>MDKNLHQPLGGNEMPRFGGIATMMRLPHVQSPAELDALDAAFVGVPLDIGTSLRSGTRFGPREIRAESVMIRPYNMATGAAPFDSLNVADIGDVAINTFNLLEAVRIIEQEYDRILGHGILPLTLGGDHTITLPILRAIKKKHGKVGLVHVDAHADVNDHMF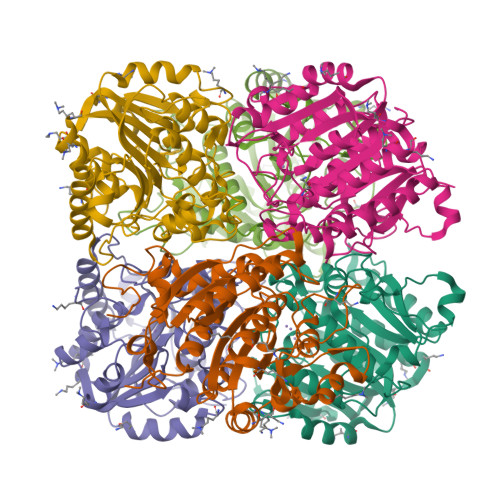GEKIAHGTTFRRAVEEDLLDCDRVVQIGLRAQGYTAEDFNWSRKQGFRVVQAEECWHKSLEPLMAEVREKVGGGPVYLSFDIDGIDPAWAPGTGTPEIGGLTTIQAMEIIRGCQGLDLIGCDLVEVSPPYDTTGNTSLLGANLLYEMLCVLPGVVRR[6x]> KFSPQLLSLLSLKTSLSGPPSAFQDWKVPVNGQNDAVWCSWSGVVCDNVTAQVISLDLSHRNLSGRIPIQIRYLSSLLYLNLSGNSLEGSFPTSIFDLTKLTTLDISRNSFDSSFPPGISKLKFLKVFNAFSNNFEGLLPSDVSRLRFLEELNFGGSYFEGEIPAAYGGLQRLKFIHLAGNVLGGKLPPRLGLLTELQHMEIGYNHFNGNIPSEFALLSNLKYFDVSNASLSGSLPQELGNLSNLETLFLFQNGFTGEIPESYSNLKSLKLLDFSSNQLSGSIPSGFSTLKNLTWLSLISNNLSGEVPEGIGELPELTTLFLWNNNFTGVLPHKLGSNGKLETMDVSNNSFTGTIPSSLCHGNKLYKLILFSNMFEGELPKSLTRCESLWRFRSQNNRLNGTIPIGFGSLRNLTFVDLSNNRFTDQIPADFATAPVLQYLNLSTNFFHRKLPENIWKAPNLQIFSASFSNLIGEIPNYVGCKSFYRIELQGNSLNGTIPWDIGHCEKLLSLNLSQNHLNGIIPWEISTLPSIADVDLSHNLLTGTIPSDFGSSKTITTFNVSYNQLIGPIPSGSFAHLNPSFFSSNEGLCGDLVGKPCN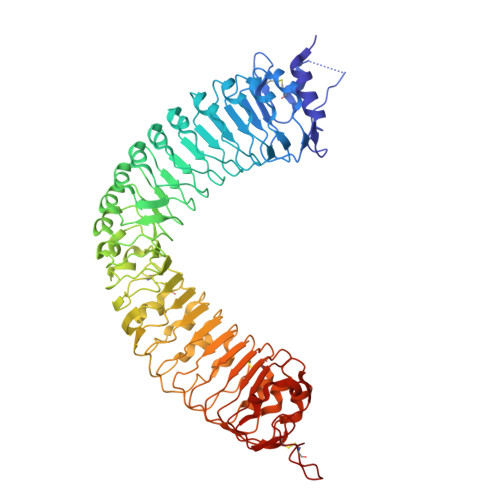SDSGLEVL> MDVSGQETDWRSTAFRQKLVSQIEDAMRKAGVAHSKSSKDMESHVFLKAKTRDEYLSLVARLIIHFRDIHNKKSQASVSDPMNALQSLTGGPAAGAAGIGMPPRGPGQSLGGMGSLGAMGQPMSLSGQPPPGTSGMAPHSMAVVSTATPQTQLQLQQVALQQQQQQQQFQQQQQAALQQQQQQQQQQQFQAQQSAMQQQFQAVVQQQQQLQQQQQQQQHLIKLHHQNQQQIQQQQQQLQRIAQLQLQQQQQQQQQQQQQQQQALQAQPPIQQPPMQQPQPPPSQALPQQLQQMHHTQHHQPPPQPQQPPVAQNQPSQLPPQSQTQPLVSQAQALPGQMLYTQPPLKFVRAPMVVQQPPVQPQVQQQQTAVQTAQAAQMVAPGVQMITEALAQGGMHIRARFPPTTAVSAIPSSSIPLGRQPMAQVSQSSLPMLSSPSPGQQVQTPQSMPPPPQPSPQPGQPSSQPNSNVSSGPAPSPSSFLPSPSPQPSQSPVTARTPQNFSVPSPGPLNTPVNPSSVMSPAGSSQAEEQQYLDKLKQLSKYIEPLRRMINKIDKNEDRKK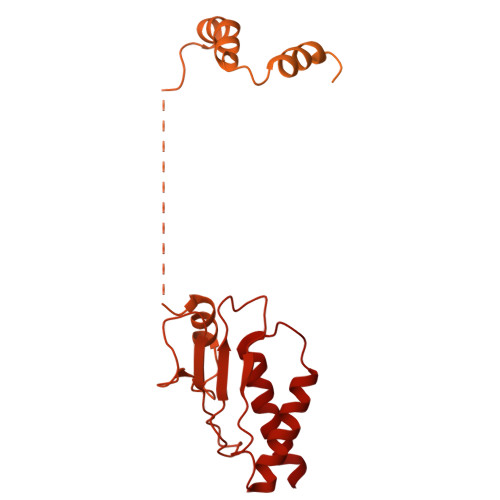DLSKMKSLLDILTDPSKRCPLKTLQKCEIALEKLKNDMAVPTPPPPPVPPTKQQYLCQPLLDAVLANIRSPVFNHSLYRTFVPAMTAIHGPPITAPVVCTRKRRLEDDERQSIPSVLQGEVARLDPKFLVNLDPSHCSNNGTVHLICKLDDKDLPSVPPLELSVPADYPAQSPLWIDRQWQYDANPFLQSVHRCMTSRLLQLPDKHSVTALLNTWAQSVHQACLSAA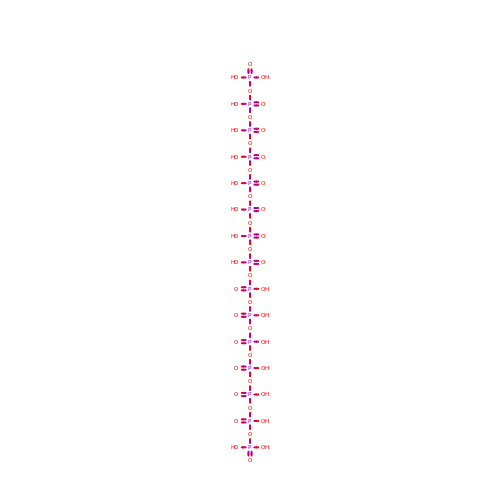pentadecaphosphate | H17 O46 P15 | NXNVLMOFLGVRFT-UHFFFAOYSA-N(~{Z})-5-[(1~{S},2~{S})-2-acetamido-1-oxidanyl-5-[oxidanyl(propanoyl)amino]pentoxy]-~{N},3-dimethyl-~{N}-oxidanyl-pent-2-enamide | C17 H31 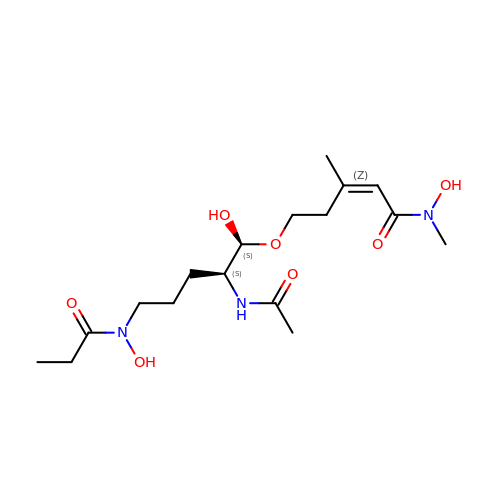N3 O7 | RTBUQAUWUAENOT-KGZSOMBESA-N>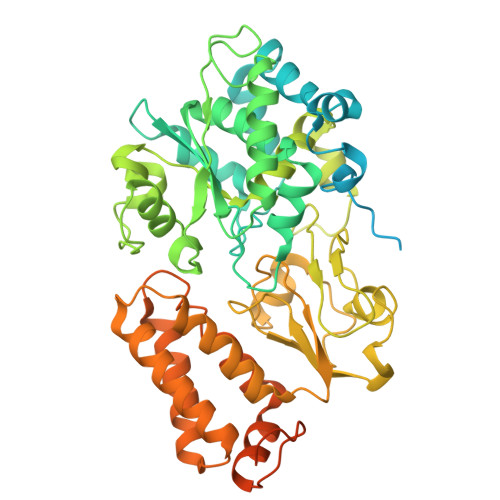 MAIYRAHVLVCRGTGCTASGAPGVMKAFKEELAKKGLDREVMLVETGCHGMCEMGPVVVVYPEGAFYCRVTPEDVPEIVEEHLYKGRIVQRLLYTVPEDMEKVPYYKDIPFYSKQHRIVLSNCGYIDPEKIEEYIARDGYMALGKALLEMTPEEVLEEVKKSGLRGRGGAGFPTGLKWEFAKKASGDKKYVICNADEGDPGAFMDRSTLEGDPHSVIEGMTIGAYVIGADEGYIYCRAEYPLAIKRLKIAIAQAEEMGLLGDHIMGTNFSFHLHLKEGAGAFVCGEETALMASIEGRRGMPRPRPPFPAQHGLWGKPTNINNVETWANVPRIILNGADWFASMGTEKSKGTKIFALTGKITNTGLIEVPMGITIREIIYELGGGILNGKEFKAVQIGGPSGGCLTKEHLDLPIDYESLTAAGAIMGSGGLVVMDEDTCMVDVAKFFLEFTQRESCGKCVPCREGTKQMLLMLQKICNGEGTMDDLSKLEELAHMVKETSLCGLGQTAPNPVITTIRYFRDEYVAHIKDKRCPAKICPALIKYVVDPEKCRKCGLCARNCPVKCISGDRQTPYLINQEKCIKCGTCMQVCPFGAIGKV>[2x]SNAMLSPEALTTAVDAAQQAIALADTLDVLARVKTEHLGDRSPLALARQALAVLPKEQRAEAGKRVNAARNAAQRSYDERLATLRAERDAAVLVAEGIDVTLPSTRVPAGARHPIIMLAEHVADTFIAMGWELAEGPEVETEQFNFDALNFPADHPARGEQDTFYIAPEDSRQLLRTHTSPVQIRTLLARELPVYIISIGRTFRTDELDATHTPIFHQVEGLAVDRGLSMAHLRGTLDAFARAEFGPSARTRIRPHFFPFTEPSAEVDVWFANKIGGAAWVEWGGCGMVHPNVLRATGIDPDLYSGFAFGMGLERTLQFRNGIPDMRDMVEGDVRFSLPFGVGA;>ENLYFQSNAMRLPYSWLREVVAVGASGWDVTPGELEQTLLRIGHEVEEVIPLGPVDGPVTVGR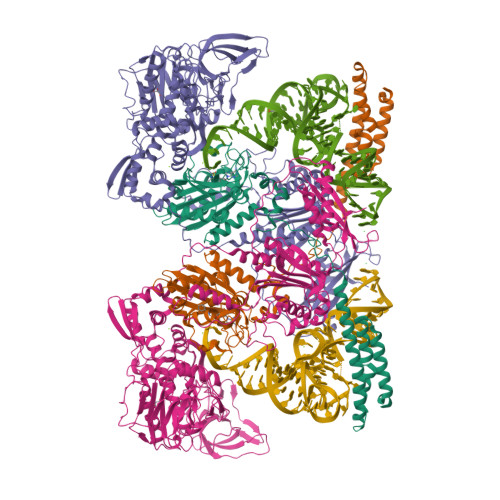VADIEELTGYKKPIRACAVDIGDRQYREIICGATNFAVGDLVVVALPGATLPGGFTISARKAYGRNSDGMICSAAELNLGADHSGILVLPPGAAEPGADGAGVLGLDDVVFHLAITPDRGYCMSVRGLARELACAYDLDFVDPASNSRVPPLPIEGPAWPLTVQPETGVRRFALRPVIGIDPAAVSPWWLQRRLLLCGIRATCPAVDVTNYVMLELGHPMHAHDRNRISGTLGVRFARSGETAVTLDGIERKLDTADVLIVDDAATAAIGGVMGAASTEVRADSTDVLLEAAIWDPAAVSRTQRRLHLPSEAARRYERTVDPAISVAALDRCARLLADIAGGEVSPTLTDWRGDPPCDDWSPPPIRMGVDVPDRIAGVAYPQGTTARRLAQIGAVVTHDGDTLTVTPPSWRPDLRQPADLVEEVLRLEGLEVIPSVLPPAPAGRGLTAGQQRRRTIGRSLALSGYVEILPTPFLPAGVFDLWGLEADDSRRMTTRVLNPLEADRPQLATTLLPALLEALVRNVSRGLVDVALFAIAQVVQPTEQTRGVGLIPVDRRPTDDEIAMLDASLPRQPQHVAAVLAGLREPRGPWGPGRPVEAADAFEAVRIIARASRVDVTLRPAQYLPWHPGRCAQVFVGESSVGHAGQLHPAVIERSGLPKGTCAVELNLDAIPCSAPLPAPRVSPYPAVFQDVSLVVAADIPAQAVADAVRAGAGDLLEDIALFDVFTGPQIGEHRKSLTFALRFRAPDRTLTEDDASAARDAAVQSAAERVGAVLRG[2x]N~2~-(PHOSPHONOACETYL)-L-ASPARAGINE 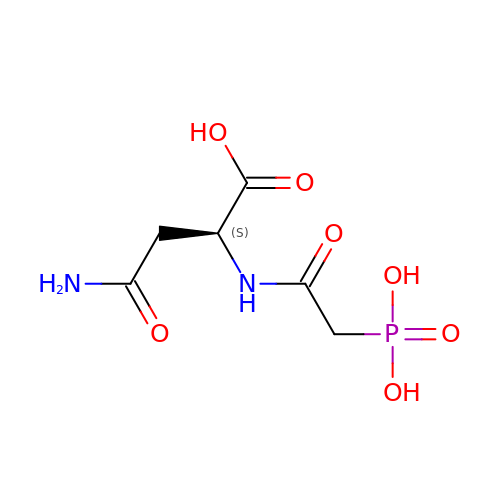| C6 H11 N2 O7 P | DDKQZYWRWCFCJX-VKHMYHEASA-N>GIPRVSEDLKDALSTFQQTFVVSDATKPDYPIMYASAGFFNMTGYTSKEVVGRNCRFLQGSGTDADELAKIRETLAAGNNYCGRILNYKKDGTSFWNLLTIAPIKDESGKVLKFIGMQVEVSKHTE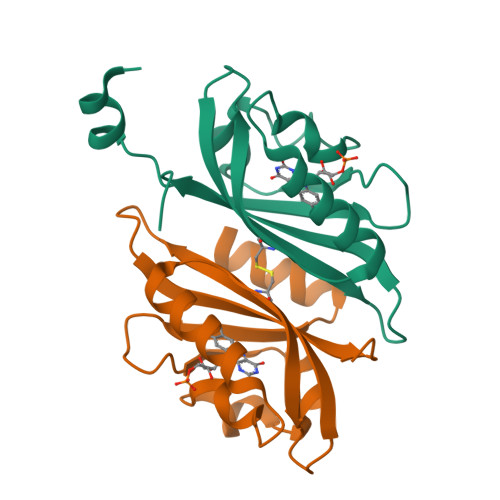GAK[2x]>[3x]MRGSH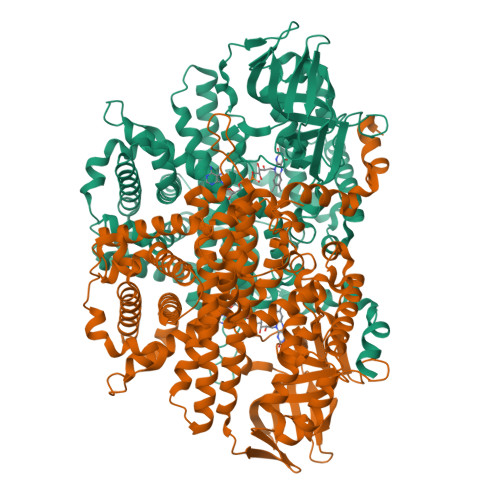HHHHHGSACELVREMEGVDYLADERKKAGFDVDEMKIVWAGSRHDFELTDRISKLVASDPGFSKEGRTMLPRKELFKNTLRKAAYAWKRIIELRLSQEEATMLRRYVDEPAFTDLHWGMFIPAIKGQGTDKQQEKWLPLAYKMQIIGCYAQTELGHGSNVQGLETTATFDPQTDEFVIHSPTLTSSKWWPGGLGKVSTHAVVYARLITDGKDYGVNGFIVQLRSLEDHKPLPGVTVGDIGMKFGNGAYNSMDNGVLSFDHVRIPRDQMLMRVSQVTKEGKYVQSDIPRQLLYGTMVYVRQSIVADASLAMSRAVCIATRYSAVRRQFGSQNGGQETQVIDYKTQQNRLFPLLASAYAFRFVGEWLKWLYTDVTQRLAANDFSTLPEAHACTAGLKSLTTSATADGIEECRKLCGGHGYLCSSGLPELFAVYVPACTYEGDNVVLQLQVARFLMKTISQLGTGKKPVGTVSYMGRIEHLMQCRSDVKQAEDWLKPSAVLEAFEARSARMSVACAKNLSKFENQEEGFAELAADLVEAAVAHCQLIVVSKYIEKLQQNIPGKGVKQQLEVLCGIYSLFILHKHQGDFLGTGYITSKQGSLANDQLRALYSQLRPNAVSLVDAFNYTDHYLGSILGRYDGNVYPKLYEAAWKDPLNKSDIADGFHEYIRPLLKQQLRTAKL> MSNTEELIQNSIGFLQKTFKALPVSFDSIRHEPLPSSMLHASVLNFEWEPLEKNISAIHDRDSLIDIILKRFIIDSMTNAIEDEEENNLEKGLLNSCIGLDFVYNSRFNRSNPASWGNTFFELFSTIIDLLNSPSTFLKFWPYAESRIEWFKMNTSVEPVSLGESNLISYKQPLYEKLRHWNDILAKLENNDILNTVKHYNMKYKLENFLSELLPINEESNFNRSASISALQESDNEWNRSARERESNRSSDVIFAADYNFVFYHLIICPIEFAFSDLEYKNDVDRSLSPLLDAILEIEENFYSKIKMNNRTRYSLEEALNTEYYANYDVMTPKLPVYMKHSNAMKMDRNEFWANLQNIKESDDYTLRPTIMDISLSNTTCLYKQLTQEDDDYYRKQFILQLCFTTNLIRNLISSDETRNFYKSCYLRENPLSDIDFENLDEVNKKRGLNLCSYICDNRVLKFYKIKDPDFYRVIRKLMSSDEKFTTAKIDGFKEFQNFRISKEKIPPPAFDETFKKFTFIKMGNKLINNVWKIPTGLDKIEQEVKKPEGVYEAAQAKWESKISSETSGGEAKDEIIRQWQTLRFLRSRYLFDFDKVNEKTGVDGLFEEPRKVEALDDSFKEKLLYKINQEHRKKLQDAREYKIGKERKKRALEEEASFPE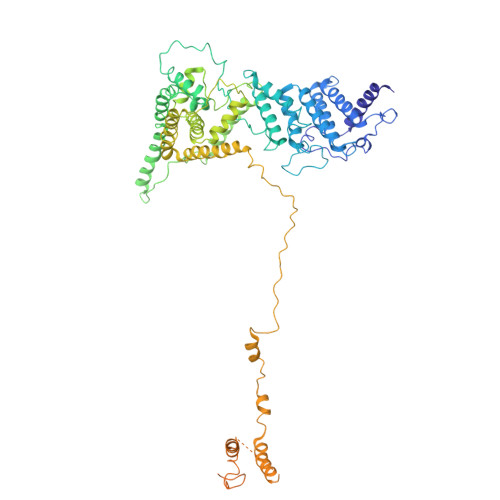REQKIKSQRINSASQTEGDELKSEQTQPKGEISEENTKIKSSEVSSQDPDSGVAGEFAPQNTTAQLENPKTEDNNAATSNISNGSSTQDMK4-aminofuran-2-carboxylic 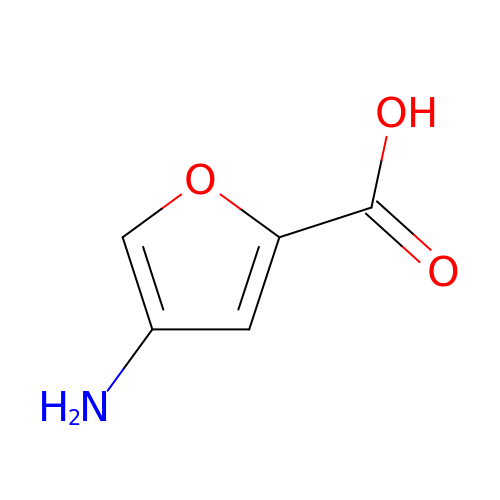acid | C5 H5 N O3 | JZMYAVSMLZDPMH-UHFFFAOYSA-N>MMDYGIDIWGNENFIIKNGKVCINYEKKPAIIDIVKELRDDGYKGPLLLRFPHLIQKQIENIYGNFNKARKEFGYKGGFNAVYPLKVNQYPGFVKNLVKLGKDYNYGLEAGSKAELLLAMAYNNEGAPITVNGFKDRELINIGFIAAEMGHNITLTIEGLNELEAIIDIAKERFKPKPNIGLRVRLHSAGVGIWAKSGGINSKFGLTSTELIEAVNLLKENKLLEQFTMIHFHLGSQITEIHPLKKALNEAGNIYTELRKMGAKNLKAINLGGGLAVEYSQFKNEKSRNYTLREYANDVVFILKNIAEQKKDLEPDIFI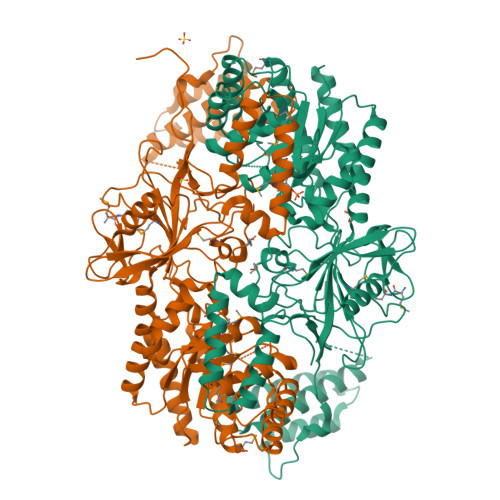ESGRFVAANHAVLIAPVLELFSQEYAENKLILKKQNPKLIDELYDLYKSIKPSNALEYLHDSIDHLESILTLFDLGYVDLQDRSNAEILTHLITKKAILLLGDKQNPADLLAIQDEVQERYLVNFSLFQSMPDFWGLEQNFPIMPLDRLDEEPTRSASIWDITCDSDGEISYSKDKPLFLHDVDVEKENYFLGFFLVGAYQEVLGMKHNLFTHPTEAIISINEKGYEVEGIIEAQSILDTLEDLDYDIHAIMDILNERISNSKLVNDKQKKHILGELYLFLNDNGYLKSIGVLEHHHHHH[2x]> SMHLICQSGDVLSARYEIVDTLGEGAFGKVVECIDHKAGGRHVAVKIVKNVDRYCEAARSEIQVLEHLNTTDPNSTFRCVQMLEWFEHHGHICIVFELLGLSTYDFIKENGFLPFRLDHIRKMAYQICKSVNFLHSNKLTHTDLKPENILFVQSDYTEAYNPKIKRDERTLINPDIKVADFGSATYDDEHHSTLVSTRHYRAPEVILALGWSQPCDVWSIGCILIEYYLGFTVFPTHDSKEHLAMMERILGPLPKHMIQKTRKRKYFHHDRLDWDEHSSAGRYVSRACKPLKEFMLSQDVEHERLFDLIQKMLEYDPAKRITLREALKHPFFDLLK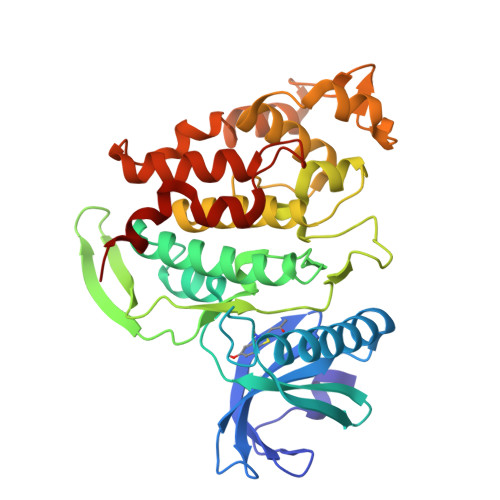KSI> MPMYEDRVDLYGADGKLLEEDVPLEAVSPLKNPTIANLVSDVKRSVAVNLAGIEGSLRKAALGGKSNFIPGREVDLPIVENAEAIAEK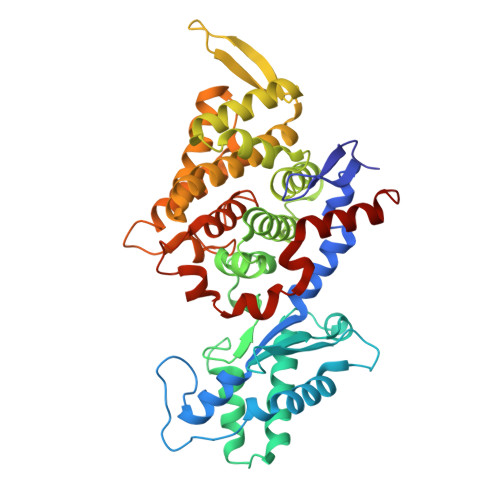IKKLVQTSEDDDTNIRLINNGQQILVQVPTTRMGVAADYTVSALVTGAAVVQAIIDEFDVDMFDANAVKTAVMGRYPQTVDFTGANLSTLLGPPVLLEGLGYGLRNIMANHVVAITRKNTLNASALSSILEQTAMFETGDAVGAFERMHLLGLAYQGLNANNLLFDLVKENGKGTVGTVIASLVERAIEDRVIKVAKEMTSGYKMYEPADWALWNAYAATGLLAATIVNVGAARAAQGVASTVLYYNDILEYETGLPGVDFGRAMGTAVGFSFFSHSIYGGGGPGIFHGNHVVTRHSKGFALPCVAAAMCLDAGTQMFSVEKTSGLIGSVYSEIDYFREPIVNVAKGAAEIKDQL> MGKLIRLELFNFKSYKGHHTLLFGDSYFTSIIGPNGSGKSNSMDAISFVLGIKSSHLRSSNLRDLIYRGRVMKTSKIQDDGTTAPATNGDVNGYENGDAGDDEDTSQRTSRNDPKTAWVMAVYEDDAGELHRWKRTITANGTSEYRINDRVVNAQQYNEALEKENILIKARNFLVFQGDVEAIASQSPQDLTRLIEQISGSLEYKEEYERLEEEVRQATEEQAYKLQRRRAANSEIKQYMEQSPGLEVLFMDRLDHVRKQLEQTEQEFEASKAKLRQARESFQAVKQKRLELFNKAFTHIQEQITHVYKELTRSEAYPLG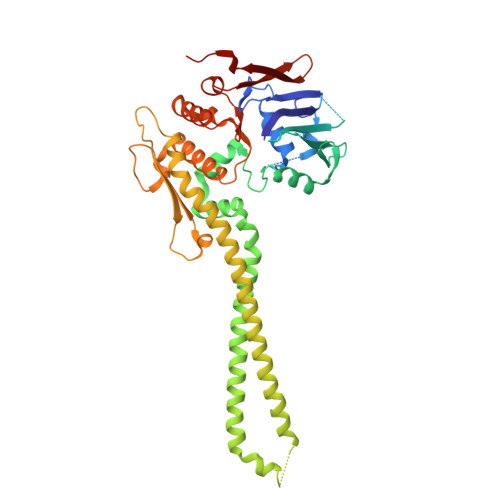GQAYLDIEEDTDTPFLSGVKYHAMPPLKRFRDMEHLSGGEKTMAALALLFAIHSYQPSPFFVLDEVDAALDNANVEKIKKYIREHAGPGMQFIVISLKPALFQASESLIGVYRDQEANTSRTLTLDLRKYRHH>[8x]PGMDSLPNPYLQSVSLTVCYMVKIKANLLSPFGKNPELQVDFGTGTGQGGDIPFRFWYCDGIVVMNTLKDGSWGKEQKLHTEAFVP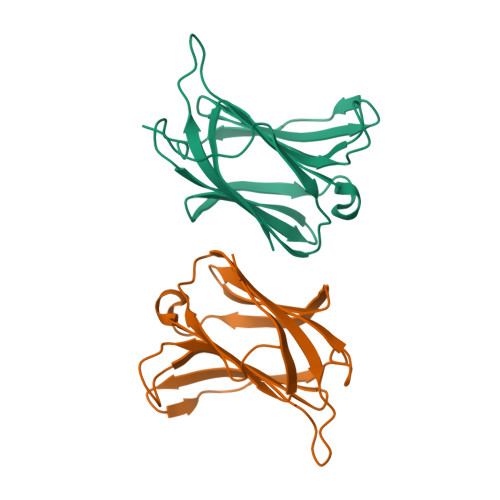GQPFELQFLVLENEYQVFVNNKPICQFAHRLPLQSVKMLDVRGDIVLTSVDTL> MGKEKSHINVVVIGHVDSGKSTTTGHLIYKCGGIDKRTIEKFEKEAAELGKGSFKYAWVLDKLKAERERGITIDIALWK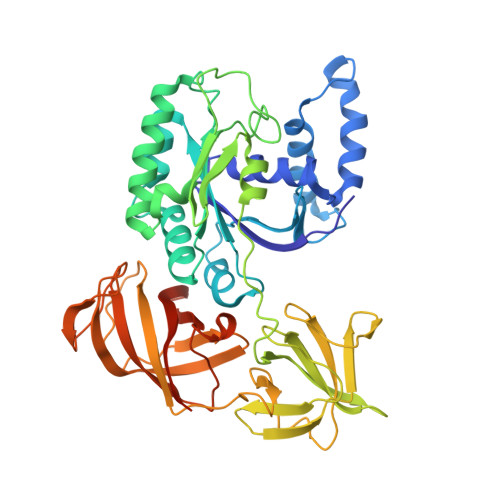FETPKYQVTVIDAPGHRDFIKNMITGTSQADCAILIIAGGVGEFEAGISKDGQTREHALLAFTLGVRQLIVAVNKMDSVKWDESRFQEIVKETSNFIKKVGYNPKTVPFVPISGWNGDNMIEATTNAPWYKGWEKETKAGVVKGKTLLEAIDAIEQPSRPTDKPLRLPLQDVYKIGGIGTVPVGRVETGVIKPGMVVTFAPAGVTTEVKSVEMHHEQLEQGVPGDNVGFNVKNVSVKEIRRGNVCGDAKNDPPKGCASFNATVIVLNHPGQISAGYSPVLDCHTAHIACRFDELLEKNDRRSGKKLEDHPKFLKSGDAALVKFVPSKPMCVEAFSEYPPLGRFAVRDMRQTVAVGVIKSVDKTEKAAKVTKAAQKAAKK>G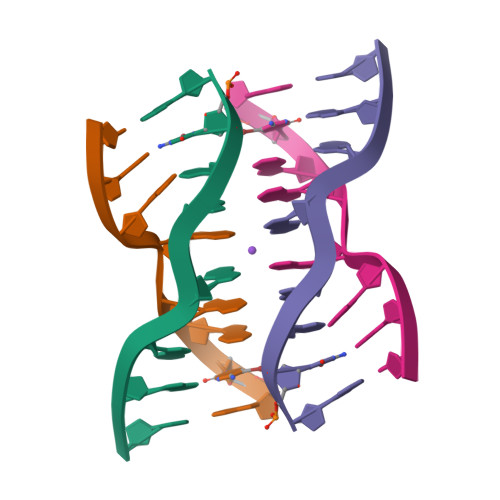CGAGAGC[2x]>[2x]AYRDQPLGELALSIPRASALFRKYDMDYAAGGKQTLARAAARKELDVEVIEAELAKLAEQPIEKDWRSAPLAEIIDHIIVRYHDRHREQLPELILQATKVERVHADKPSVPKGLTKYLTMLHELLSSHMMKEEQILFPMIKQGMGSQAMGPISVMESEHDEAGELLEVIKHTTNNVTPPPEACTTWKAMYNGINELIDDLMDHISLENNVLFPRALAGE

Escherichia coli YtfE is a di-iron protein of the widespread Repair of Iron Centers proteins (RIC) family that has the capacity to donate iron, which is a crucial component of the biogenesis of the ubiquitous family of iron-sulfur proteins. Bacterial RICs are composed by an N-terminal ScdA-like domain and a C-terminal domain that folds as a four-helix bundle where a histidine/carboxylate di-iron type center is inserted. In E. coli YtfE, the best studied RIC protein, the center is coordinated by H84, H129, H160, H204, and two μ-carboxylate bridges formed by E133 and E208. We show that YtfE establishes protein-protein interactions with the scaffold IscU, where the transient cluster is formed, and the cysteine desulfurase IscS.

The mutation of E125 (which is located at ca. 9 Å from its nearest iron in the di-iron center) to leucine generated a protein with an intact binuclear site. Escherichia coli YtfEM and YtfEM-E125L contain a di-iron site coordinated by four histidine residues, through their Nε2 atoms (H84 and H204 for Fe1, H129 and H160 for Fe2), and two bidentate glutamic acids that bridge the two irons (E133, E208). The mutation in YtfEM-E125L induced a major modification of the channel. In this case, a significant shortening of the distance between the sidechains of residues L125 and E159 is observed, from 8.5 Å in YtfEM to 5.3 Å in YtfEM-E125L. As a consequence, the new position of L125 results in the occlusion of the channel and, consequently, the di-iron center is no longer exposed to the solvent. The closing of the channel is consistent with the different iron release properties of the YtfEM-E125L, and explains why this mutant protein is no longer able to promote the formation of the Fe-S center in IscS. In particular, the ferric dissociation constant of YtfE is substantially modified by the E125L mutation, becoming about 4-fold larger than that determined for the wild-type protein. Mutation of E125 to asparagine decreased the V0 values by about 3-fold whereas a leucine substitution reduced the iron-release rate by ca. 8-fold. On the contrary, the spectra of the reaction mixtures containing IscU and YtfE-E125N or IscU and YtfE-E125L exhibited very weak bands, which indicates that the amount of ISC formed in IscU is negligible. However, and unexpectedly, the YtfE-E125L mutant has a hindered capacity to release iron and is not able to promote the assembly of the iron-sulfur center in IscU. These results were rationalized by the analysis of the crystal structure of YtfEM-E125L showing that the positioning of the L125 sidechain blocks the external part of the hydrophilic channel, and consequently impairs the release of iron from the di-iron cluster to protein exterior.(5R)-1-methyl-7-[5-(propan-2-yloxy)pyridin-3-yl]-1,7-diazaspiro[4.4]nonane 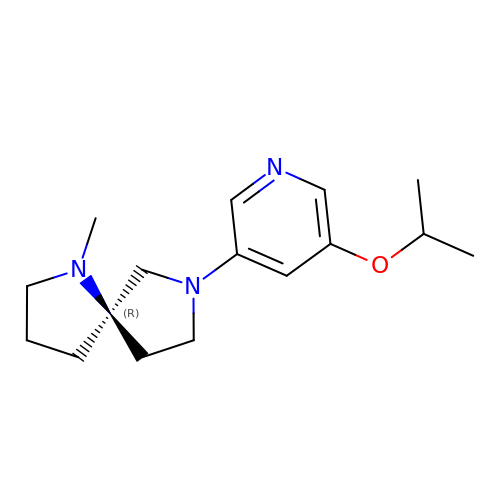| C16 H25 N3 O | KVSRTRCOWRKRQB-MRXNPFEDSA-N>AEQKTLHIYNWTDYIAPDTVANFEKETGIKVVYDVFDSNEVLEGKLMAGSTGFDLVVPSAYLLERQLTAGVFQPLDKSKLPEWKNLDPELLKLVAKHDPDNKFAMPYMWATTGIGYNVDKVKAVLGENAPVDSWDLILKPENLEKLKSCGVSFLDDPEEVFATVLNYLGKDPNSTKADDYTGPATDLLLKLRPNIRYFHSSQYINDLANGDICVAIGWAGDVWQASNRAKEA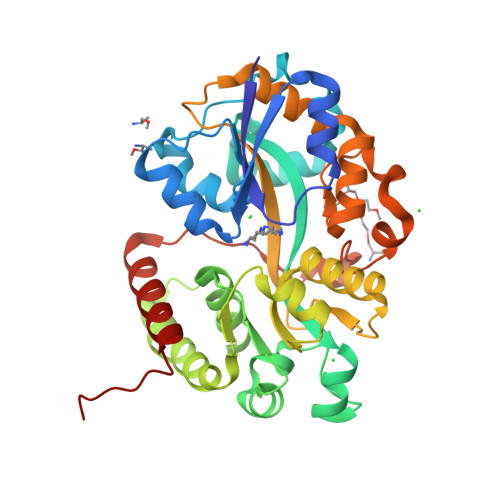KNGVNVSFSIPKEGAMAWFDVFAMPADAKNKDEAYQFLNYLLRPDVVAHISDHVFYANANKAATPLVSAEVRENPGIYPPADVRAKLFTQKVQDPKIDRVRTRAWTKVKSGKLEHHHHHH[2x]The soluble guanylyl cyclase (sGC) is a heterodimeric enzyme that, upon activation by nitric oxide, stimulates the production of the second messenger cGMP. Each sGC subunit harbor four domains three of which are used for heterodimerization: H-NOXA/H-NOBA domain, coiled-coil domain (CC), and catalytic guanylyl cyclase domain. The CC domain has previously been postulated to be part of a larger CC family termed the signaling helix (S-helix) family. Dimerization within sGC is mediated by at least three inter-domain interactions involving the GC, H-NOXA/H-NOBA, and CC subdomains.

We determined the crystal structure of the Rattus norvegicus sGC CC domain (residues A348-K409) to 2.15 Å resolution using SeMet single-anomalous-dispersion (SAD)-phasing. Crystals were initially obtained of the wt sequence but the SAD phasing required the introduction of an additional Met residue via the I371 M mutation. The I371 M mutation that was generated for SeMet phasing is not involved in the dimer or tetramer interface. There are 8 CC molecules in the asymmetric unit and each monomer contains a long amphipathic a helix aA with 13 helical turns followed by a turn and a short helix aB. The turn is initiated by a conserved proline residue, P399. Four sGC CC monomers come close together to form an apparent four-helix bundle in an anti-parallel arrangement with two of such tetramers in the asymmetric unit. The CC monomers A and B (and the equivalent CD, EF, and GH) form an anti-parallel CC dimer. The side-chain directions of a-helices follow a heptad (a-g) repeat in that residue i and i+7 face the same direction. The CC dimer interface is formed predominantly via the a-d pattern residues and the a-d assignment, as obtained from SOCKET, is indicated in Figure 1B.

>GSHMATRDLVLLGEQFREEYKLTQELEMLTDRLQLTLRALEDEKKKTDTLLYSVLPPSVANELRHK[8x]> GAQVSTQKTGAHETGLNASGNSIIHYTNIN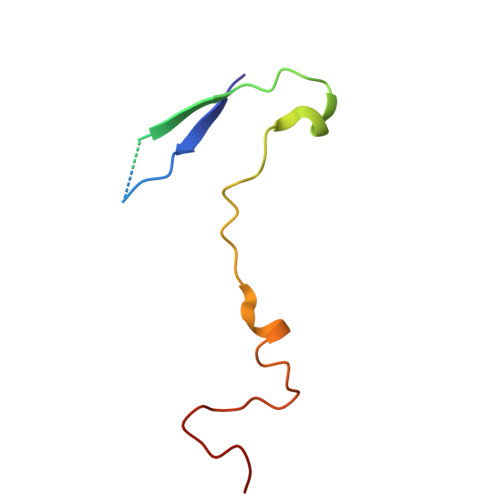YYKDAASNSANRQDFTQDPGKFTEPVKDIMIKSLPALN> HHHHHHMAEVKLYGFWPSPFSHRIIWALKLKGVEYEYIEEDLSNKSESLLKYNPVYKKIPVLVHGDKPIAESLVILEYIEETWPENPLLPKDPYERAMARFWIQYGVDTVAALRAFYLGSGEELEKAAKELSECLKILEEQGLGDKKFFGGESMNLVDISYGALGYWLAAVEEAKGVTVLKP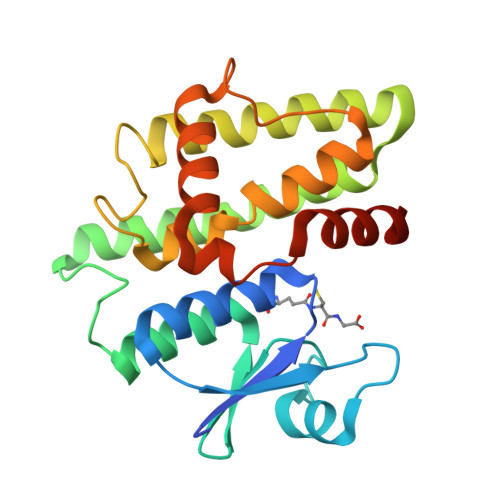STLPRLHAWAKNLDELPVVKENIPASDKMLAYVTAAMNRPAKN>[2x]MASKIEQPRWASKDSAAGAASTPDEKIVLEFMDALTSNDAAKLIEYFAEDTMYQNMPLPPAYGRDAVEQTLAGLFTVMSIDAV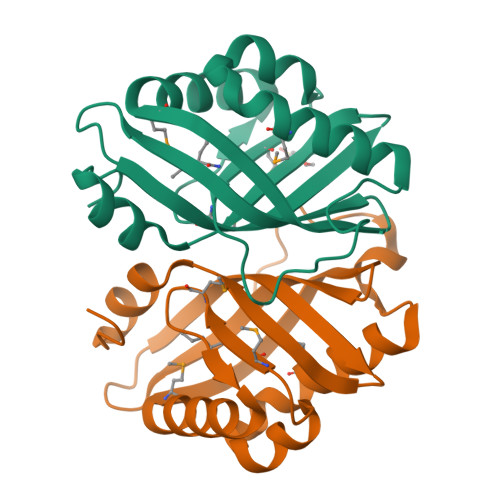ETFHIGSSNGLVYTERVDVLRALPTGKSYNLSILGVFQLTEGKITGWRDYFDLREFEEAVDLPLRG>[2x]MTDPNSPYFEKVLGSLFARQVEPAKDYAWDMGSTLPTPDDLMRRFIVKDTLITIFRRHGAVEAPTATLYPKSSHYGPNAVHLLDRNGTVLQLPFDLVMGHARSLARIASGPVPQRAYSFGNIFRDRQDGGQPDVYGEVDFDIVTTDAMDLAMKEAEVIKVLDEIIAAFPTTSSTPMCFQLGHSDLLQLIFDFCNVEHGARQAAA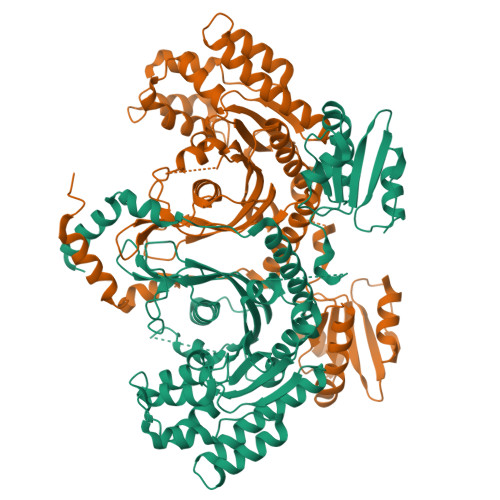EVLSKLNIRNFTWQKVRSELRSPLVGISATSVDELQRFDWRDTPTKAFTKIRNLFEGTEYYDKVSSTLAHLKEVYEYSKKFKVNTKIYIAPLSSINEAFFRGGILFSCLYDRKVMDVFAAGGRYDGLIKAHRPRIGSRFEERHAVGFSLNWEKQLAKPVPKTTGKAFLKKAAEEEAQGIFSAKRCDVLVASFDPSILRSSGIELLQMLWAHGISAELARDARSPEDLLTTYRDESYSWIVIIKQESQLKIKTMHRKDVPDADIQAKDLLAWLKAEI> MKKAVINGEQIRSISDLHQTLKKELALPEYYGENLDALWAALTGWVEYPLVLEWRQFEQSKQLT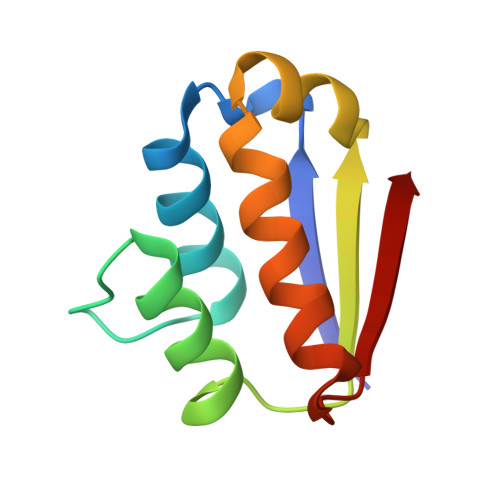ENGAESVLQVFREAKAEGADITIILS> MSLTRRDFVKLCTGTVAGFGISQMFHPAVHEALAGTLTGERPPVFWLQGQGCTGCSVTLLNSVHPSIADVLLKVISLEFHPTVMAWEGEHAIEHMRKVAEKFKGKFFLVIEGSVPVEADGKYCIIGEANHHEISMVDALKEFGPNAAAVLAVGTCAAYGGIPAAEGSETGATAVSKFLGDNGIKTPVVNIPGCPPHPDWIVGTVVLALDAIKKNGLEGGLAEVVKVLDSDGRPTPFFGRNIHENCPYLDKYDEGVMSATFTDKVGCRYDLGCKGPMTMADCFERKWNGGVNWCVQNAVCIGCVEPDFPDGKSPF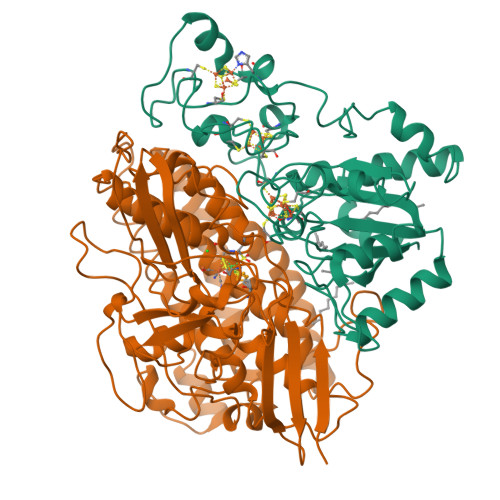YQA;> MSGCTPKAAPAGATGRTTIAIDPVTRIEGHLKAEVVVENGKVVDARLSGGMYRGFETILRGRDPRDASQIVQRICGVCPTAHSTASVLALDEAFGAKVPNNGRITRNLIFGANYLQSHILHFYHLSAQDFVQGPDTAPFVPRFPKSDLRLSKELNKAGVDQYIEALEVRRICHEMVALFGGRMPHVQGQVVGGATEIPTKEKLVEYAARFKKVRDFVEQKYVPVVYTIGSKYKDMFKVGQGFKAALCVGAFPLDNSGKKHLFMPGVYAKGKDMPFDPSKIKEYVKYSWFAEETTGLNYKEGKTIPAPDKAGAYSFVKAPRYDGLSLEVGPLARMWVNNPELSPVGKKLLKDLFGISAKKFRDLGEEAAFSLMGRHVARAEETYYMLGAIEGWLKEIKAGEDTVVMPAVPASAEGTGFTEAPRGSLLHYVKVKDSKIDNYQIVSASLWNCNPRDDMGQRGAVEEALIGIPVDDIQNPVNVARLIRAFDPULGCAVH(2S,4S)-1-[(2S)-2-amino-2-cyclohexylacetyl]-4-fluoropyrrolidine-2-carbonitrile 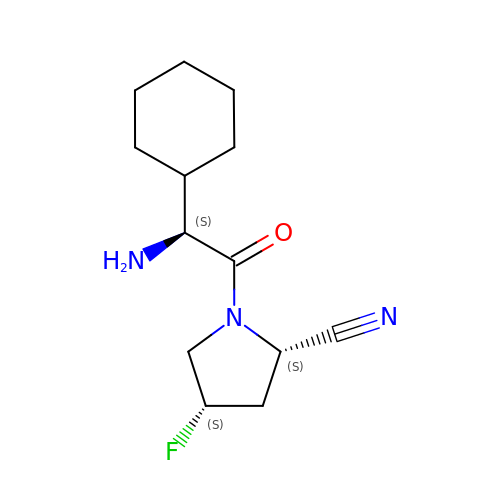| C13 H20 F N3 O | PITTXTFNBYNBSG-SRVKXCTJSA-N>SMAEIKQGIREVILCKDQDGKIGLRLKSIDNGIFVQLVQANSPASLVGLRFGDQVLQINGENCAGWSSDKAHKVLKQAFGEKITMTIRDRPFERTITMHKDSTGHVGFIFKNGKITSIVKDSSAARNGL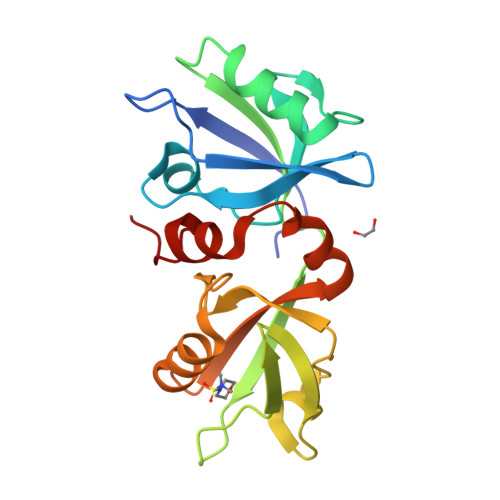LTEHNICEINGQNVIGLKDSQIADILSTSGTVVTITIMPAFIFEHIIKRMAPSIMKSLMDHTIPEV[4x]In the present work, we identified deoxycytidine kinase (dCK) as the target responsible for the sensitisation of various cancer cell lines to gemcitabine, using reverse-proteomics. dCK is a key enzyme in the nucleoside salvage pathway and recycles bases and nucleosides originating from the degradation of RNA and DNA to achieve the biosynthesis of deoxyribonucleotides, which are required for DNA replication and repair. This cytosolic nucleoside kinase catalyses the 5′-phosphorylation of 2′-deoxycytosine (2′dC), 2′-deoxyadenosine (2′dA) and 2′-deoxyguanosine (2′dG). dCK is also responsible for the initial phosphorylation of numerous anticancer and antiviral nucleoside analogues. dCK adds the first phosphoryl group to nucleosides analogues and is usually the rate-limiting enzyme of the overall process of converting nucleosides to their deoxynucleoside triphosphate form. Hence, dCK is clinically important because of its relationship to both drug resistance and sensitivity. Previous work has revealed that dCK can adopt several distinct conformations, which are a function of the nature of the nucleoside and nucleotide bound.

In order to understand this activation mechanism, we solved crystal structures of dCK in complex with masitinib/UDP and imatinib/UDP. We found that the masitinib pyridine ring mimics a pyrimidine base in the nucleoside binding site, while the rest of the molecule extends to a cavity only available in the ‘open’ conformation of dCK. For both molecules, interactions with dCK mainly involve non-polar interactions, without direct polar interactions. Additionally, for each ligand-bound structure, a supplementary electron density was present at the top of the cavity, likely corresponding to a second molecule of compound interacting weakly with the first one in a similar binding mode as the ‘F-series’ inhibitors reported previously. Moreover, it should be noted that masitinib and imatinib were able to open dCK in situ, since we were able to obtain these 3D structures in the ‘open’ conformation by soaking the protein kinase inhibitors in a ‘closed’ dCK crystal. The binding of these compounds also released the monophosphorylated substrate (2′-deoxycytidine-5′-monophosphate), observed in the ‘closed’ dCK crystal and still present in the other nucleoside binding site subunit, elucidating at the same time its mechanism of action. Furthermore, our structural data revealed that binding of masitinib or imatinib promotes and maintains an open conformation of dCK, critical for the release of products and the subsequent nucleoside binding. In contrast, our structures show that TKIs binds partially at the active site, but without strong direct hydrogen bond interactions and without sterically interfering with the catalytic residues.

>MSYYHHHHHHLESTSLYKKAGLENLYFQGMATPPKRSSPSFSASSEGTRIKKISIEGNIAAGKSTFVNILKQLSEDWEVVPEPVARWSNVQSTQDEFEELTMSQKNGGNVLQMMYEKPERWSFTFQTYACLSRIRAQLASLNGKLKDAEKPVLFFERSVYSDRYIFASNLYESECMNETEWTIYQDWHDWMNNQFGQSLELDGIIYLQATPETCLHRIYLRGRNEEQGIPLEYLEKLHYKHESWLLHRTLKTNFDYLQEVPILTLDVNEDFKDKYESLVEKVKEFLSTL[4x]7,8-dihydroxy-4-phenyl-2H-chromen-2-one | 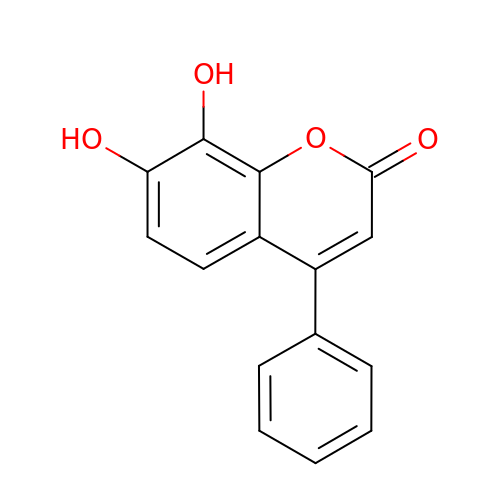C15 H10 O4 | JRVIIPJSVKTPBK-UHFFFAOYSA-N> IAELPPKVSVFVPPRDGFFGNPRKSKLICQATGFSPRQIQVSWLREGKQVGSGVTTDQVQAEAKESGPTTYKVTSTLTIKESDWLGQSMFTCRVDHRGLTFQQNASSMCVPDQDTAIRVFAIPPSFASIFLTKSTKLTCLVTDLTTYDSVTISWTRQNGEAVKTHTNISESHPNATFSAVGEASICEDDWNSGERFTCTVTHTDLPSPLKQTISRPKGVALHRPDVYLLPPAREQLNLRESATITCLVTGFSPADVFVQWMQRGQPLSPEKYVTSAPMPEPQAPGRYFAHSILTVSEEEWN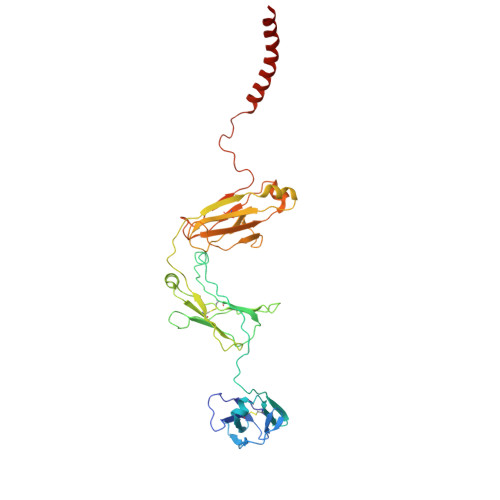TGETYTCVVAHEALPNRVTERTVDKSTEGEVSADEEGFENLWATASTFIVLFLLSLFYSTTVTLF>GHMASVTRAVFGELPSGGGTVEKFQLQSDLLRVDIISWGCTITALEVKDRQGRASDVVLGFAELEGYLQKQPYFGAVIGRVANRIAKGTFKVDGKEYHLAINKEPNSLHGGVRGFDKVLWTPRVLSNGVQFSRISPDGEEGYPGELKVWVTYTLDGGELIVNYRAQASQATPVNLTNHSYFNLAGQASPNINDHEVTIEADTYLPVDETLIPTGEVAPVQGTAFDLRKPVELGKHLQDFHLNGFDHNFCL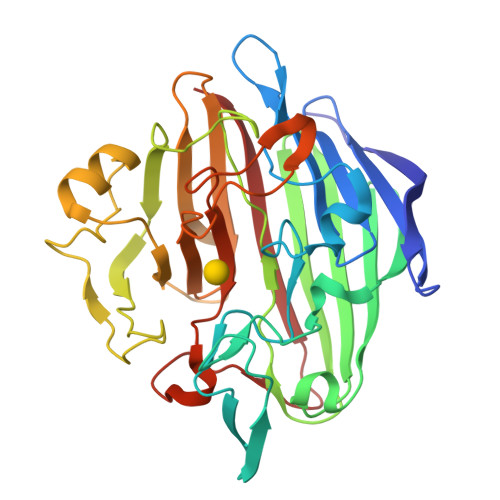KGSKEKHFCARVHHAASGRVLEVYTTQPGVQFYTGNFLDGTLKGKNGAVYPKHSGFCLETQNWPDAVNQPRFPPVLLRPGEEYDHTTWFKFSVA[4x]> NTSLEAIVQNASSDNQGIQLSAVQAARKLLSSDRNPPIDDLIKSGILPILVHCLERDDNPSLQFEAAWALTNIASGTSEQTQAVVQSNAVPLFLRLLHSPHQNVCEQAVWALGNIIGDGPQCRDY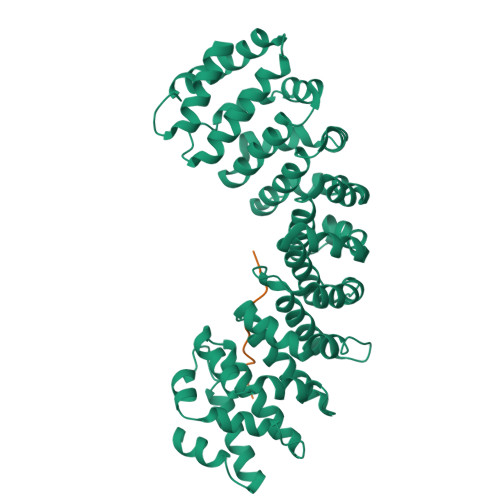VISLGVVKPLLSFISPSIPITFLRNVTWVMVNLCRHKDPPPPMETIQEILPALCVLIHHTDVNILVDTVWALSYLTDAGNEQIQMVIDSGIVPHLVPLLSHQEVKVQTAALRAVGNIVTGTDEQTQVVLNCDALSHFPALLTHPKEKINKEAVWFLSNITAGNQQQVQAVIDANLVPMIIHLLDKGDFGTQKEAAWAISNLTISGRKDQVAYLIQQNVIPPFCNLLTVKDAQVVQVVLDGLSNILKMAEDEAETIGNLIEECGGLEKIEQLQNHENEDIYKLAYEIIDQFF;> GSSPEGGEDSDREDGNYCPPVKRERTSSLT>SGGNYTKFDVKNWVRREHFEFYRHRLPCGFSLTSKIDITTLKKSLDDSAYKFYPVMIYLIAQAVNQFDELRMAIKDDELIVWDSVDPQFTVFHQETETFSALSCPYSSDIDQFMVNYLSVMERYKSDTKLFPQGVTPENHLNISALPWVNFDSFNLNVANFTDYFAPIITMA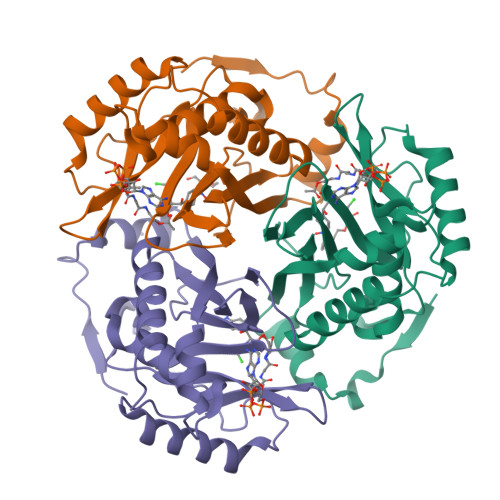KYQQEGDRLLLPLSVQVHHAVCDGFHVARFINRLQELCNSKLK[3x]> MRKFNSHSIPIRLNLLFSIVILLFMTIIGRLLYMQVLNKDFYEKKLASASQTKITSSSARGEIYDASGKPLVENTLKQVVSFTRSNKMTATDLKETAKKLLTYVSISSPNLTERQLADYYLADPEIYKKIVEALPSEKRLDSDGNRLSESELYNNAVDSVQTSQLNYTED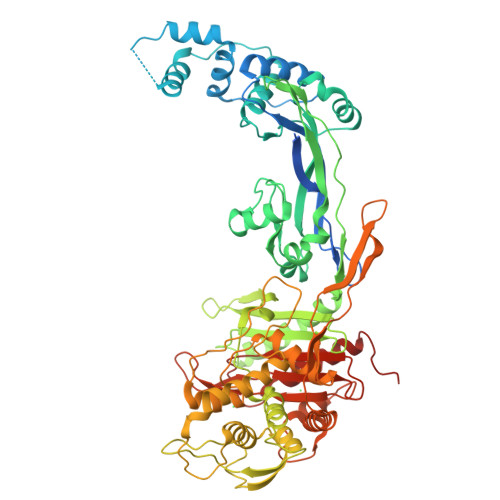EKKEIYLFSQLNAVGNFATGTIATDPLNDSQVAVIASISKEMPGISISTSWDRKVLETSLSSIVGSVSSEKAGLPAEEAEAYLKKGYSLNDRVGTSYLEKQYEETLQGKRSVKEIHLDKYGNMESVDTIEEGSKGNNIKLTIDLAFQDSVDALLKSYFNSELENGGAKYSEGVYAVALNPKTGAVLSMSGIKHDLKTGELTPDSLGTVTNVFVPGSVVKAATISSGWENGVLSGNQTLTDQSIVFQGSAPINSWYTQAYGSFPITAVQALEYSSNTYMVQTALGLMGQTYQPNMFVGTSNLESAMEKLRSTFGEYGLGTATGIDLPDESTGFVPKEYSFANYITNAFGQFDNYTPMQLAQYVATIANNGVRVAPRIVEGIYGNNDKGGLGDLIQQLQPTEMNKVNISDSDMSILHQGFYQVAHGTSGLTTGRAFSNGALVSISGKTGTAESYVADGQQATNTNAVAYAPSDNPQIAVAVVFPHNTNLTNGVGPSIARDIINLYQKYHPMNHH> HHHHHHSSGLVPRGSHM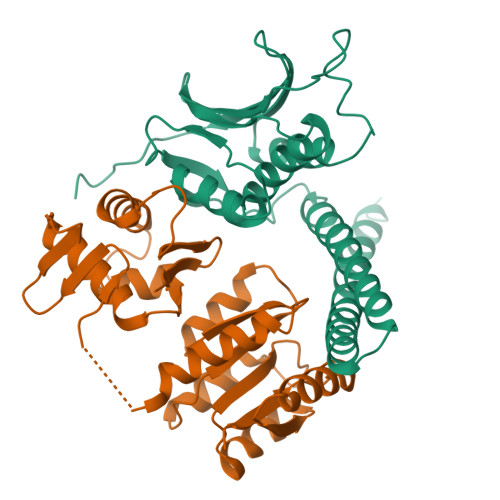EQIRNALLAALSHDLRTPLTVLFGQAEILTLDLASEGSPHARQASEIRQHVLNTTRLVNNLLDMARIQSGGFNLKKEWLTLEEVVGSALQMLEPGLSSPINLSLPEPLTLIHVDGPLFERVLINLLENAVKYAGAQAEIGIDAHVEGENLQLDVWDNGPGLPPGQEQTIFDKFARGNKESAVPGVGLGLAICRAIVDVHGGTITAFNRPEGGACFRVTLPQQTAPELEEFHEDM;> HHHHHHSSGLVPRGSHMTNVLIVEDEQAIRRFLRTALEGDGMRVFEAETLQRGLLEAATRKPDLIILDLGLPDGDGIEFIRDLRQWSAVPVIVLSARSEESDKIAALDAGADDYLSKPFGIGELQARLRVALRRHSATTAPDPLVKFSDVTVDLAARVIHRGEEEVHLTPIEFRLLAVLLNNAGKVLTQRQLLNQVWGPNAVEHSHYLRIYMGHLRQKLEQDPARPRHFITETGIGYRFML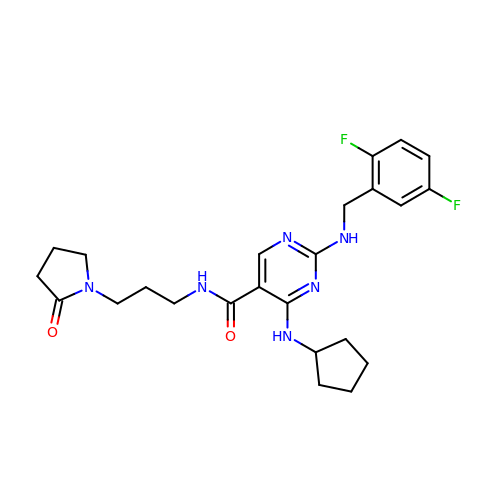2-[[2,5-bis(fluoranyl)phenyl]methylamino]-4-(cyclopentylamino)-N-[3-(2-oxidanylidenepyrrolidin-1-yl)propyl]pyrimidine-5-carboxamide | C24 H30 F2 N6 O2 | CGCYACANDHXNLI-UHFFFAOYSA-N>[2x]GSEAAGGEQRELLIQRLRAAVHYTTGALAQDVAEDKGVLFSKQTVAAISEITFRQAENFARDLEMFARHAKRSTITSEDVKLLARRSNSLLKYITQKSDELASSNME;>[2x]GYEEREGGFRKETVERLLRLHFRDGRTRVNGDALLLMAELLKVFVREAAARAARQAQAEDLEKVDIEHVEKVLPQLLLDFV;> GRSLHHKSALFSCVTDPKEMHCHENWSLSPEEFEIWDRL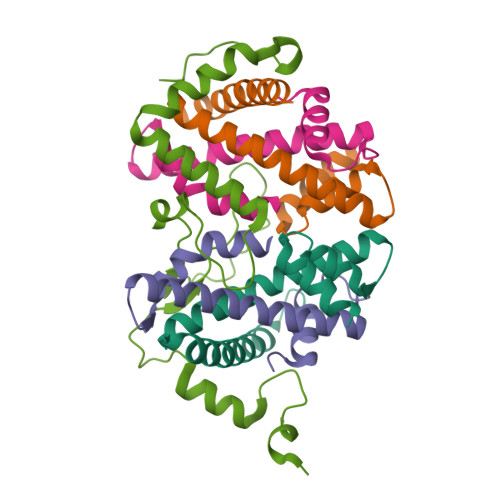YRLKENDGVKEPILPHTRFETLENLDKTSKPEEEAAHKLSLSEWSIWQSRPFPTSMVDHSDRCYHFISVMELIEVMRQEQGDCSYELELQPHLRIEDIHVRRNKGHLSP> NGDRLYRADSRPPDEIKRSGGLMPRGHNEYFDRGTQMNINLYDHA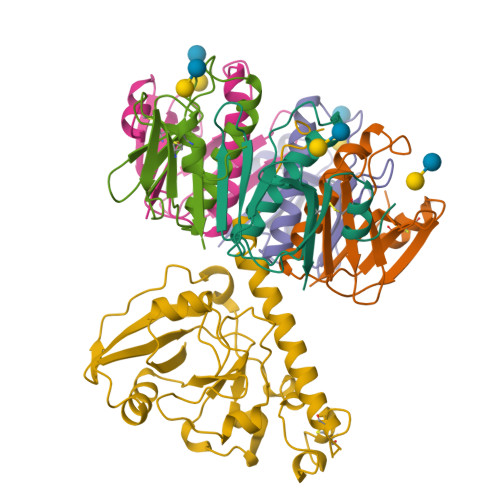RGTQTGFVRYDDGYVSTKLSLRSAHLAGQSILSGYSTYYIYVIATAPNMFNVNDVLGVYSPHPYEQEVSALGGIPYSQIYGWYRVNFGVIDERLHRNREYRDRYYRNLNIAPAEDGYRLAGFPPDHQAWREEPWIHHAPQGCGNSSNSSRTITRTITGDTCNEETQNLSTIYLREYQSKVKRQIFSDYQSEVDIYNRIRDEL;>[5x]APQTITELCSEYRNTQIYTINDKILSYTESMAGKREMVIITFKSGETFQVEVPGSQHIDSQKKAIERMKDTLRITYLTETKIDKLCVWNNKTPNSIAAISMKN> SGFNHVKPTEYKPRLLHISGDKNAKVAEVPLATSSLNSGDCFLLDAGLTIYQFNGSKSSPQEKNKAAEVARAIDAE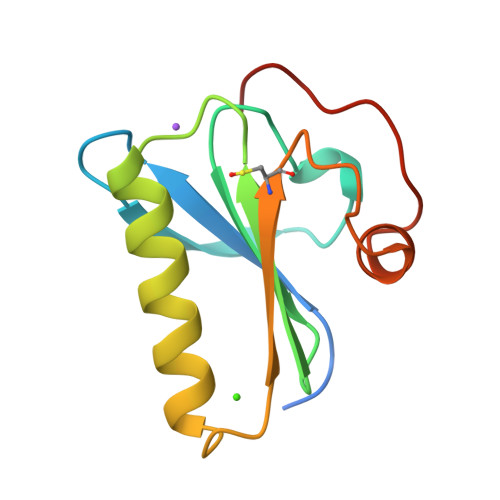RKGLPKVEVFCETDSDIPAEFWKLLGGKGAIAAKHETA>[2x]GPLGSVPPTIEQKTRAFTVPNIPLQTLSNSRFPSLIQGMILSPDASQVVQFQNGRCLIDGQLLGTTPATSGQLFRVRGKINQGARTLNLTEVDGKPFMAFDSPAPVGFPD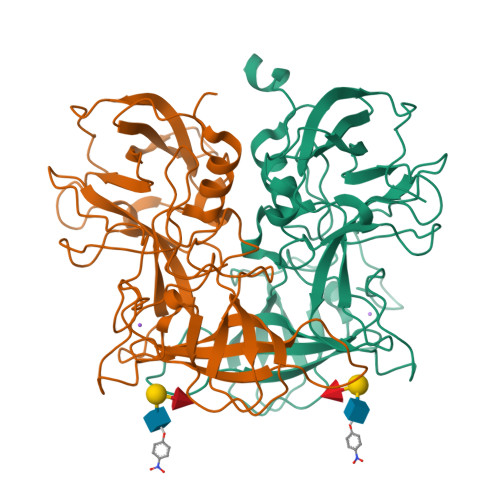FGKCDWHMRISKTPNNTSSGDPMRSVSVQTNVQGFVPHLGSIQFDEVFNHPTGDYIGTIEWISQPSTPPGTDINLWEIPDYGSSLSQAANLAPPVFPPGFGEALVYFVSAFPGPNNRSAPNDVPCLLPQEYITHFVSEQAPTMGDAALLHYVDPDTNRNLGEFKLYPGGYLTCVPNGVGAGPQQLPLNGVFLFVSWVSRFYQLKPVGTASTARSRL>[2x]G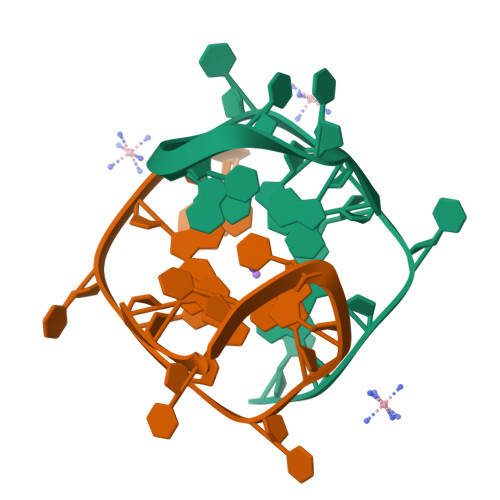GCTCGGCGGCGGA> IVRPPFTYATLIRQAIMESSDRQLTLNEIYSWFTRTFAYFRRNAAT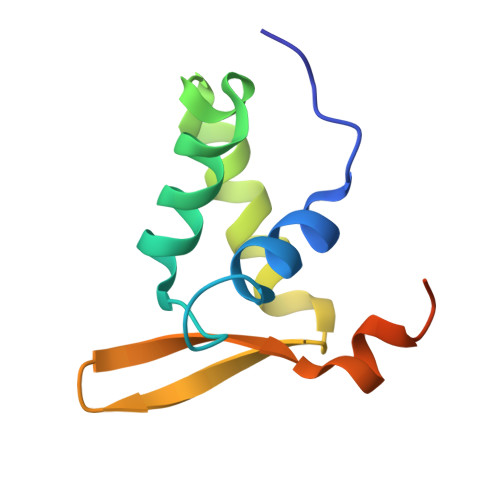WKNAVRHNLSLHKCFVRVENVKGAVWTVDEVEYQKRRSQKITGSPTL>[2x]GSHMEQLKHCNGILKELL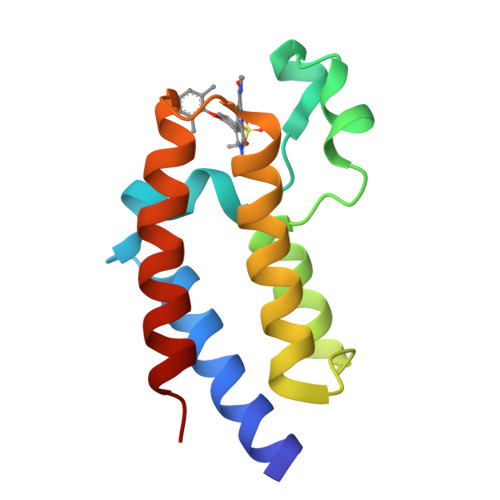SKKHAAYAWPFYKPVDASALGLHDYHDIIKHPMDLSTVKRKMENRDYRDAQEFAADVRLMFSNCYKYNPPDHDVVAMARKLQDVFEFRYAKMPD>[6x]MAHHHHHHDDDKMMSASKEIKSFLWTQSLRRELSGYCSNIKLQVVKDAQALLHGLDFSEVSNVQRLMRKERRDDNDLKRLRDLNQAVNNLVELKSTQQKSILRVGTLTSDDLLILAADLEKLKSKVIRTERPLSAGVYMGNLSSQQLDQRRALLNMI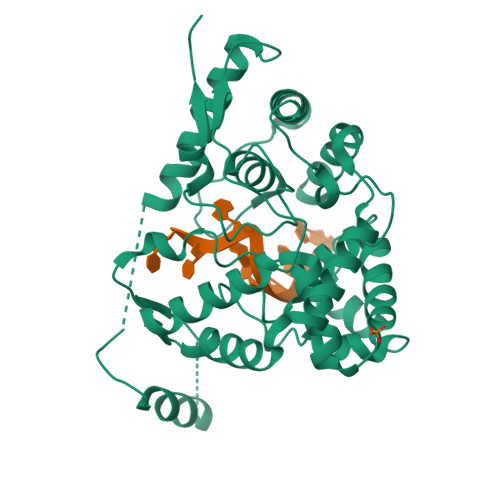GMSGGNQGARAGRDGVVRVWDVKNAELLSNQFGTMPSLTLACLTKQGQVDLNDAVQALTDLGLIYTAKYPNTSDLDRLTQSHPILNMIDTKKSSLNISGYNFSLGAAVKAGACMLDGGNMLETIKVSPQTMDGILKSILKVKKALGMFISDTPGERNPYENILYKICLSGDGWPYIASRTSITGRAWENTVVDLES>MTIGIDKINFYVPKYYVDMAKLAEARQVDPNKFLIGIGQTEMAVSPVNQDIVSMGANAAKDIITDEDKKKIGMVIVATESAVDAAKAAAVQIHNLLGIQP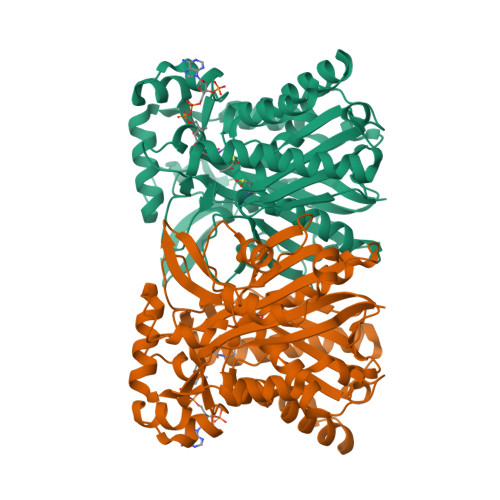FARCFEMKEACYAATPAIQLAKDYLATRPNEKVLVIATDTARYGLNSGGEPTQGAGAVAMVIAHNPSILALNEDAVAYTEDVYDFWRPTGHKYPLVDGALSKDAYIRSFQQSWNEYAKRQGKSLADFASLCFHVPFTKMGKKALESIIDNADETTQERLRSGYEDAVDYNRYVGNIYTGSLYLSLISLLENRDLQAGETIGLFSYGSGSVVEFYSATLVEGYKDHLDQAAHKALLNNRTEVSVDAYETFFKRFDDVEFDEEQDAVHEDRHIFYLSNIENNVREYHRPE[4x]>MVQAPSVYVCGFVERPDAPPKDACLHLDPLTVKSQLPLKKPLPLTVEHLPDAPVGSVFGLYQSSAGLFSAASITSGDFLSLLDSIYHDCDIAQSQRLPLPREPKVEALHAWLPSLSLASLHPDIPQTTADGGKLSFFDHVSICALGRRRGTTAVYGTDLAWVLKHFSDLEPSIAAQIENDANAAKRESGCPEDHPLPLTKLIAKAIDAGFLRNRVETLRQDRGVANIPAESYLK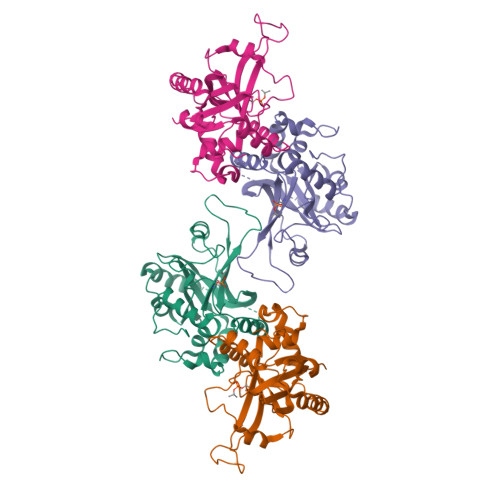A[2x]>[4x]MAKDIGINSDPNSSSVDKLMKSSGVSNPTYTLVWKVWILAVTLYYAI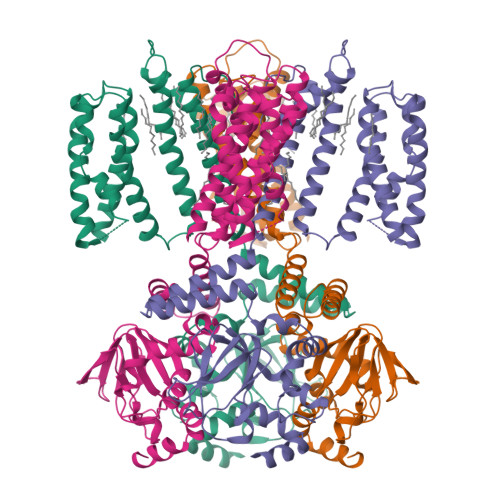RIPLTLVFPSLFSPLLPLDILASLALIADIPLDLAFESRRTSGRKPTLLAPSRLPDLLAALPLDLLVFALHLPSPLSLLSLVRLLKLISVQRSATRILSYRINPALLRLLSLVGFILLAAHGIACGWMSLQPPSENPAGTRYLSAFYWTITTLTTIGYGDITPSTPTQTVYTIVIELLGAAMYGLVIGNIASLVSKLDAAKLLHRERVERVTAFLSYKRISPELQRRIIEYFDYLWETRRGYEEREVLKELPHPLRLAVAMEIHGDVIEKVPLFKGAGEEFIRDIILHLEPVIYGPGEYIIRAGEMGSDVYFINRGSVEVLSADEKTRYAILSEGQFFGEMALILRAPRTATVRARAFCDLYRLDKETFDRILSRYPEIAAQIQELAVRRKELESSGLVPRGSVKHHHH> DQYEYKYPAIKDLKKPCITLGKAPDLNKAYKSVLSGMNAAKLDPDDVCSYLAAAMQFFEGTCPEDWTSYGILIARKGDRITPNSLVEIKRTDVEGNWALTGGMELTRDPTVSEHASLVGLLLSLYRLSKISGQNTGNYKTNI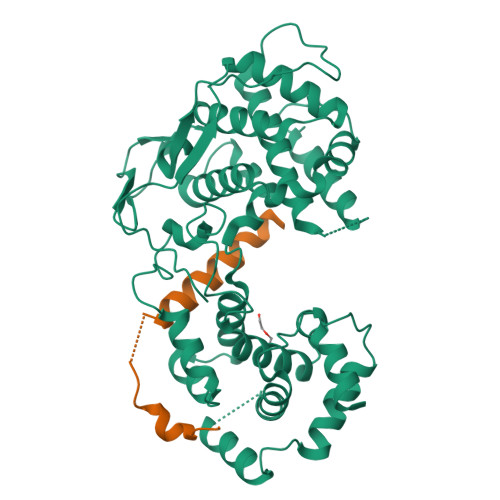ADRIEQIFETAPFVKIVEHHTLMTTHKMCANWSTIPNFRFLAGTYDMFFSRIEHLYSAIRVGTVVTAYEDCSGLVSFTGFIKQINLTAREAILYFFHKNFEEEIRRMFEPGQETAVPHSYFIHFRSLGLSGKSPYSSNAVGHVFNLIHFVGCYMGQVRSLNATVIAACAPHEMSVLGGYLGEEFFGKGTFERRFFRDEKELQEYEAAELTKSDVALADDGTVNSDDEDYFSGETRSPEAVYTRIMMNGGRLKRSHIRRYVSVSSNHQARPNSFAEFLNKTYSNDS;> MSKIFVNPSAIRAGLADLEMAEETVDLINRNIEDNQAHLQGEPIEVDNLPEDMGRLHLDGGKSPNPGELEHHHHHH> SMGGRRAVRVWCDGCYDMVHYGHSNQLRQARAMGDYLIVGVHTDEEIAKHKGPPVFTQEERYKMVQAIKWVDEVVPAAPYVTTLETLDKYNCDFCVHGNDITLTVDGRDTYEEVKQAGRYRECKRTQGVSTTDLVGRMLLVTKAHHSSQEMSSEYREYADSFGKCPGGRNPWTGVSQFLQTSQKIIQFASGKE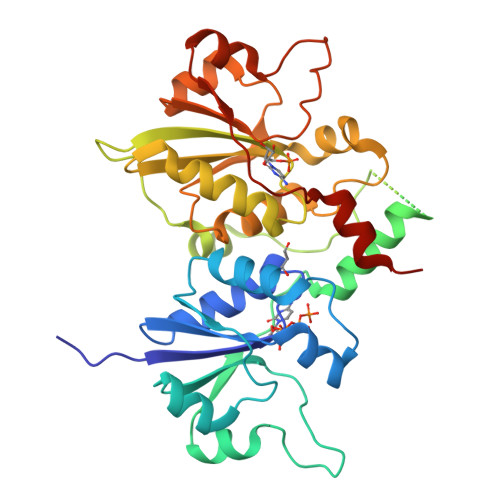PQPGETVIYVAGAFDLFHIGHVDFLEKVHRLAERPYIIAGLHFDQEVNHYKGKNYPIMNLHERTLSVLACRYVSEVVIGAPYAVTAELLSHFKVDLVCHGKTEIIPDRDGSDPYQEPKRRGIFRQIDSGSNLTTDLIVQRIITNRLEY>[3x]MRIVAADTGGAVLDESFQPVGLIATVAVLVEKPYKTSKRFLVKYADPYNY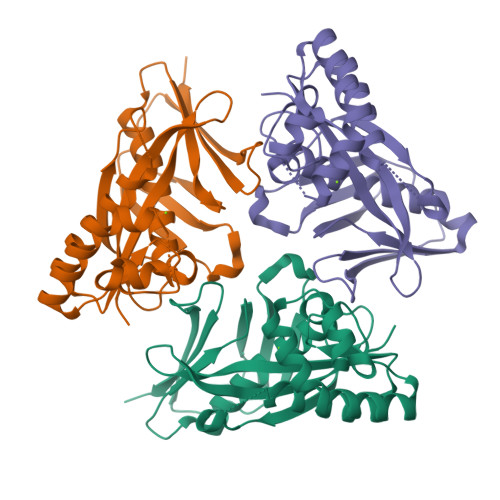DLSGRQAIRDEIELAIELAREVSPDVIHLDSTLGGIEVRKLDESTIDALQISDRGKEIWKELSKDLQPLAKKFWEETGIEIIAIGKSSVPVRIAEIYAGIFSVKWALDNVKEKGGLLVGLPRYMEVEIKKDKIIGKSLDPREGGLYGEVKTEVPQGIKWELYPNPLVRRFMVFEITSKS>[8x]MSRKPSGLGRGLEALLPKTGAGVVRLPLASIRPNPRQPRKR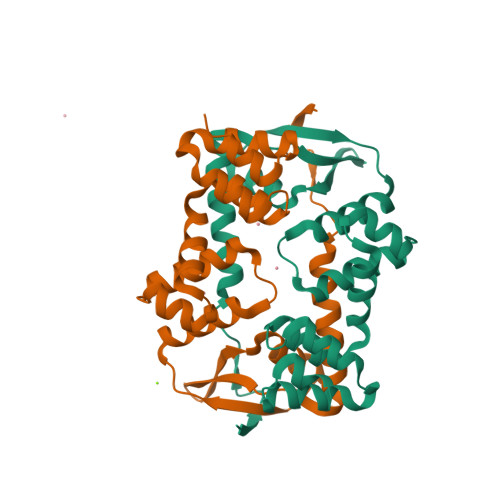FAEESLKELADSIREKGLLQPLLVRPQGDGYELVAGERRYRAALMAGLQEVPAVVKDLTDREALELALVENLQREDLSPVEEARGYQALLEMGLTQEEVARRVGKARSTVANALRLLQLPPEALEALERGEITAGHARALLMLEPEDRLWGLKEILEKGLSVRQAEALRERLAMAPKRSAEGSHHHHHH MGME1 (also known as DDK1) is a highly conserved, mitochondria-specific DNase. Human MGME1 (HsMGME1) protein is composed of 344 amino acids and belongs to the PD-(D/E)XK nuclease superfamily. However, in contrast to DNA2 (2–5) and many other mitochondrial DNases, MGME1 can cleave various types of DNA substrates with a preference for single-stranded DNAs (ssDNA). Structural analysis and comparison suggest that MGME1 follows a two-cation-assisted catalytic mechanism of substrate cleavage.

The apo-HsMGME1 structure belongs to the P43212 space group and contains one HsMGME1 molecule per asymmetric unit; the monomeric state of HsMGME1 is consistent with our gel filtration profile and a previous report. In the apo-HsMGME1 structure, residues 1–97, 113–117 and 190–198 are disordered; the β3–α5 connecting loop (aa 255–264) resides right under the helical arch. The side chain of Phe261 forms a weak hydrophobic stacking interaction with the side chains of Trp152 and Lys153 of α2; the backbone O atoms of Lys257 and Pro258 form water-mediated hydrogen bond (H-bond) interactions with Tyr168 and Thr169 of α3, respectively. These interactions may help stabilize the conformation of both the helical arch and the β3-α5 connecting loop. Though Mg2+ was not present in either the crystallization sample or the crystallization buffer, the crystallization buffer of the apo-HsMGME1 crystals contained 100 mM Mn2+. Two well-defined Mn2+ ions were captured at the active site of the apo-HsMGME1 structure, which was hereafter referred to as HsMGME1-Mn2+. In addition to three water molecules and the side chain OE2 atom of Glu344 (the last residue of HsMGME1), the B-site Mn2+ was also coordinated by TLA and Asp238, via their O1 and OD1 atoms, respectively. The average coordinating distances of the A-site and B-site Mn2+ ions were all ∼2.15 Å. Unlike many nucleases, which coordinate Mg2+ (or Mn2+) through the side chains of three or more negatively charged residues (Asp or Glu), HsMGME1 coordinates Mn2+ through the side chains of His180, Asp238, and Asp251, and the main chain of Trp252. In the HsMGME1–Mn2+ structure, the C-terminal residues 337–344 of HsMGME1 are well ordered and fold directly back into the active center.

> GEDRRVPQNWFPIFNPERSDKPNASDPSVPLKIPLQRNVIPSVTRVLQQTMTKQQVFLLERWKQRMILELGEDGFKEYTSNVFLQGKRFHEALESILSPQETLKERDENLLKSGYIESVQHILKDVSGVRALESAVQHETLNYIGLLDCVAEYQGKLCVIDWKTSEKPKPFIQSTFDNPLQVVAYMGAMNHDTNYSFQVQCGLIVVAYKDGSPAHPHFMDAELCSQYWTKWLLRLEEYTEKKKNQNIQKPEYSE> MDSINTRIAEELSALPSGRVQPQQVAAAVALLDEGSTVPFIARYRKEVTGSLDDTQLRMLEERLRYLRELEERRGAILASIEEQGKLTPELARDIKLADTKTRLEDLYLPYKQKRRTKGQIALEAGLGALADALFDDPTLVPESEAARFVDAEKGFADVKAVLEGAKYILMERFAEDATLLDKLRVFMKNEATLTARVVPGKEQEGAKFSDYFEHDEPLKSAPSHRALAIFRGRNEGVLSASLKVGEEAPGTLHPCEVMIAERFGLSNQGRAADKWLAEVVRWTWKVKLYTHLETDLFGELRDGAEDEAISVFARNLHDLLLAAPAGP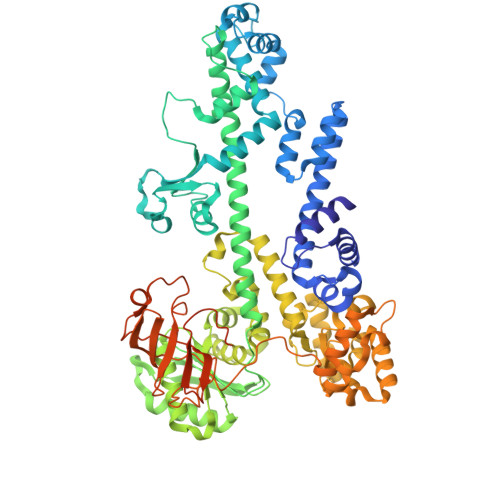RATLGLDPGLRTGVKVAVVDATGKLLDTATVYPHAPKNQWDQTLAVLAALCAKHQVELIAIGNGTASRETDKLAGELIKKYPGMKLTKIMVSEAGASVYSASELAAKEFPELDVSLRGAVSIARRLQDPLAELVKIEPKSIGVGQYQHDVSQLKLARSLDAVVEDCVNAVGVDVNTASAALLARISGLNSTLAQNIVAHRDANGAFRTRDELKKVSRLGEKTFEQAAGFLRVMNGDNPLDASAVHPETYPLVQRIAADTERDIRSLIGDSAFLKRLDPKKFTDETFGLPTVTDILKELDKPGRDPRPEFKTAEFQEGVESLKDLKPGMVLEGVVTNVTNFGAFVDIGVHQDGLVHISALSEKFVKDPYEVVKAGDIVKVKVMEVDIPRNRVGLSMRMSDTPGEKVEGQRGGRPTGSGQPRQERGAPRGQSAPPANNAMAALFANAKQLKKKHHHHHH> MTELCPVYAPFFGAIGCASAIIFTSLGAAYGTAKSGVGICATCVLRPDLLFKNIVPVIMAGIIAIYGLV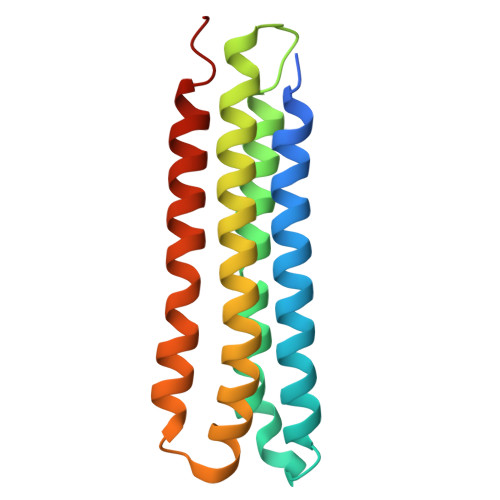VSVLVCYSLGQKQALYTGFIQLGAGLSVGLSGLAAGFAIGIVGDAGVRGSSQQPRLFVGMILILIFAEVLGLYGLIVALLLNSRATQDVVC>DTASDAAAAAALTAANAKAAAELTAANAAAAAAAT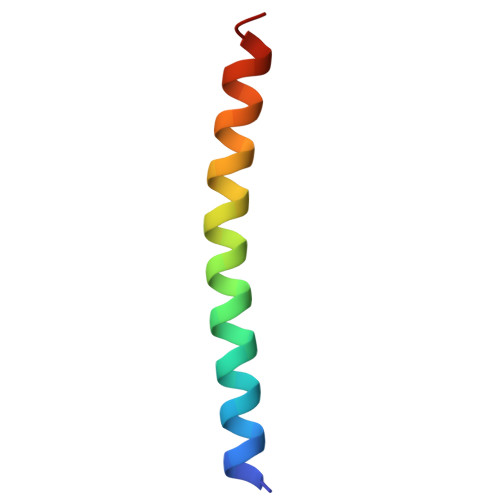ARX[2x]>SNATDTAEQVIASFRILASDKPYILAEELRRELPPDQAQY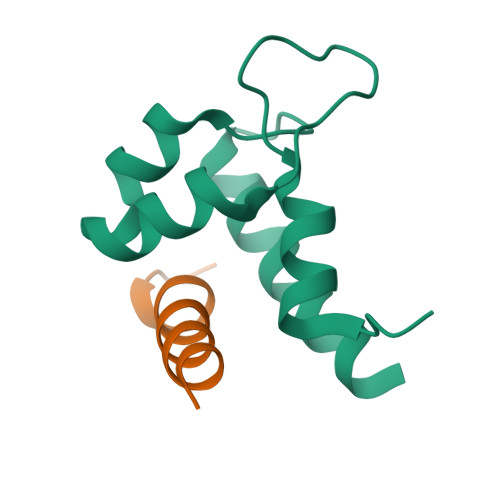CIKRMPAYSGPGSVPGALDYAAFSSALYGESDL[2x];>[2x]NARRKLKGAILTTMLATRNFSG>[3x]MSSKPKPIEIIGAPFSKGQPRGGVEKGPAALRKAGLVEKLKETEYNVRDHGDLAFVDVPNDSPFQIVKNPRSVGKANEQLAAVVAETQKNGTISVVLGGDNSMAIGSISGHARVHPDLCVIWVDAHTDINTPLTTSSGNLHGQPVAFLLKELKGKFPDVPGFSWVTPCISAKDIVYIGLRDVDPGEHYIIKTLGIKYFSMTEVDKLGIGKVMEETFSYLLGRKKRPIHLSFDVDGLDPVFTPAT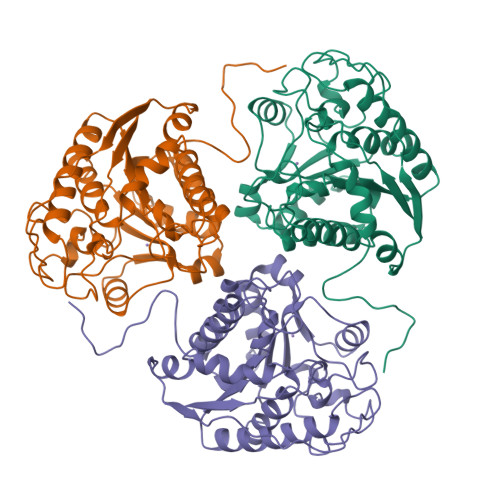GTPVVGGLSYREGLYITEEIYKTGLLSGLDIMEVNPTLGKTPEEVTRTVNTAVALTLSCFGTKREGNHKPETDYLKPPK>SNAKKEPACFSTVIPGWFSEMSPMWPGEAHSLKVEKVLFQGKSDYQDVIVFQSATYGKVLVLDGVIQLTERDECAYQEMITHLPLCSIPNPKKVLVIGGGDGGVLREVARHASIEQIDMCEIDKMVVDVSKQFFPDVAIGYEDPRVNLVIGDGVAFLKNAAEGSYDAVIVDSSDPIGPAKELFEKPFFQSVARALRPGGVVCTQAESLWLHMDIIEDIVSNCREIFKGSVNYAWTSVPTYPSGVIGFMLCSTEGPDVDFKHPLNPIDESSSKSNGPLKFYNAEIHSAAFCLPSFAKKVIESKAN[8x]

Longer polyamines are produced by aminopropyltransferases (APTs), enzymes that catalyze the transfer of an aminopropyl group from decarboxylated S-adenosylmethionine (dc-SAM), a universal cofactor of APTs, to a polyamine substrate. Thus, spermidine synthase (SPDS) utilizes PUT as the substrate for spermidine (SPD) biosynthesis. AtSPDS1 and AtSPDS2 share the fold of polyamine biosynthesis proteins with the characteristic two-domain topology. The active site of AtSPDS is formed between the N-terminal and C-terminal domains.

The third determined structure is the crystal complex of AtSPDS1 with two bound compounds, dc-SAM and CHA, which precisely shows the binding mode of the cofactor and the inhibitor of SPDS. The adenosine moiety of the dc-SAM is stacked between Leu212/216 and Ile152/156 and it forms three hydrogen bonds with the surrounding residues. Two of these H-bonds are created by the N6 amine with the carbonyl oxygen atom of Pro208/212 and the OD1 oxygen atom of Asp182/186. The third hydrogen bond is created between the N1 of dc-SAM and the backbone amide of Gly183/187. The niche is formed by polar residues, Asp131/135, Asp201/205, and Gln107/111 that create three hydrogen bonds with terminal amine of the cofactor’s aminopropyl moiety. The key residues in this part of the active site are easily recognized in the structure of AtSPDS1-CHA, where the polyamine groove is occupied by the inhibitor. CHA is bound close to two perpendicularly situated Tyr residues, Tyr106/110 and Tyr270/274, and its amine group crates three hydrogen bonds with acidic residues at the bottom of the polyamine grove. These are the direct hydrogen bond with Asp208, and the two water-mediated H-bonds with Glu236/240 and Glu50/54. The AtSPDS1-CHA structure gave insights into the inhibition of the plant SPDSs by CHA. This competitive inhibitor binds inside the polyamine groove of the active site creating three hydrogen bonds at the bottom of the pocket, analogical to these created by the bound substrate.>MKVGIDAGGTLIKIVQEQDNQRTFKTELTKNIDQVVEWLNQQQIEKLCLTGGNAGVIAENI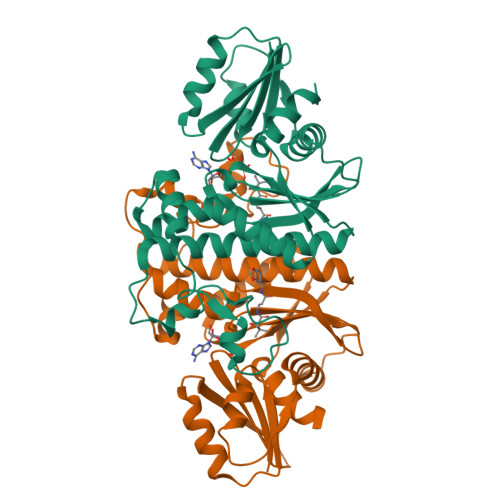NIPAQIFVEFDAASQGLGILLKEQGHDLADYIFANVGTGTSLHYFDGQSQRRVGGIGTGGGMIQGLGYLLSQITDYKQLTDMAQHGDRNTIDLKVRHIYKDTEPPIPGDLTAANFGHVLHHLDADFTPSNKLAAVIGVVGEVVTTMAITVAREFKTENIVYIGSSFHNNALLRKVVEDYTVLRGCKPYYVENGAFSGAIGALYLE[4x]>[3x]MKSEIIAVGTEILTGQIVNTNSQFLSEKFAELGIDVYFQTAVGDNEERLLSVLKIAKERSDLIVLCGGLGPTEDDLTKQTLAKFLKRELVFDKTAQERLDEFFASRPTSMRTPNNECQAQIIAGSQPLSNKTGLAVGGLLEADGVTYVVLPGPPSELKPMVNKELLPYLSKTSEKLYSRVLRFFGIG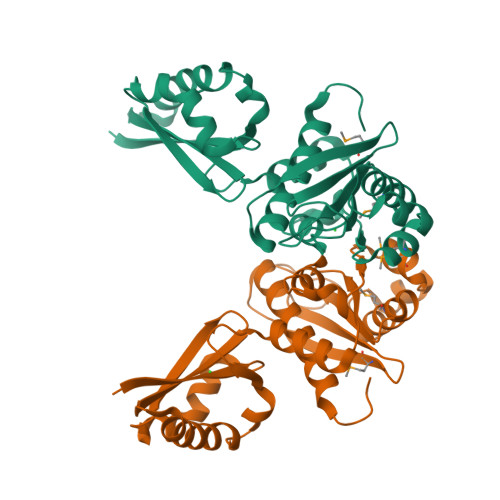ESHLVTLLHDLIAEQTDPTIAPYAKTGEVTIRLSTKAHRQKEADSKLDKLEKKIITIDNLADYFYGYGEENSLPQVVFDLLKEKGKTITAAESLTAGLFQARLADFAGASDIFKGGFITYSIEEKARMLGIPFEDLQLHGVVSAFTAEKMAERSRQLTQADLAISLTGVAGPDSLEGQPAGTVFIGLSSSKRTMAIKVLIGGRSRSDVRYIAVLHAFNLVRQTLLSHKNLV> SAKDE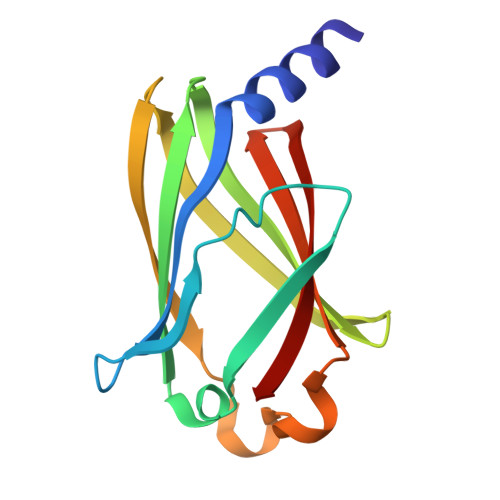RAREILRGFKLNWMNLRDAETGKILWQGTEDLSVPGVEHEARVPKKILKCKAVSRELNFSSTEQMEKFRLEQKVYFKGQCLEEWFFEFGFVIPNSTNTWQSLIEAAPESQMMPASVLTGNVIIETKFFDDDLLVSTSRVRLFYV(2~{R})-4-methyl-2-[(1~{S})-1-sulfanylethyl]pentanoic 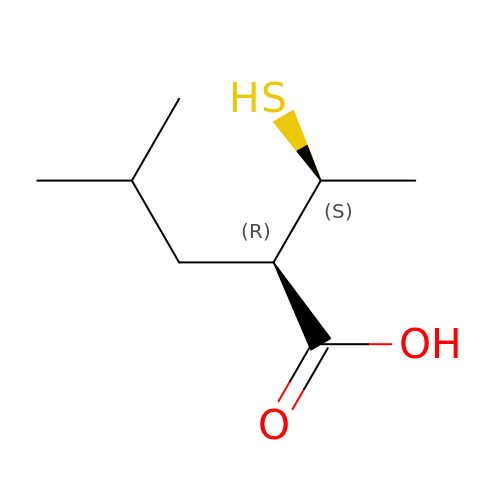acid | C8 H16 O2 S | SKKLDDQIMOJPLA-BQBZGAKWSA-N> MGSS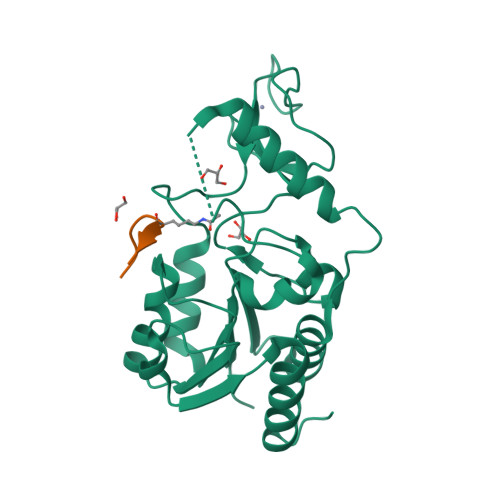HHHHHHSQDPKPRVLVLTGAGISAESGIRTFRAADGLWEEHRVEDVGTPEGFDRDPELVQAFANARRRQLQQPEIQPNAAHLALAKLQDALGDRFLLVTQNLDNLHERAGNTNVIHMHGELLKVRCSQSGQVLDWTGDVTPEDKCHCCQFPAPLRPHYVWFGEMPLGMDEIYMALSMADIFIAIGTSGHVYPAAGFVHEAKLHGAHTVELNLEPSQVGNEFAEKYYGPASQVVPEFVEKLLKGLKAGSIA;> KGGAKRHRKIL> GMGEKLELRLKSPVGAEPAVYPWPLPVYDKHHDAAHEIIETIRWVCEEIPDLKLAMENYVLIDYDTKSFESMQRLCDKYNRAIDSIHQLWKGTTQPMKLNTRPSTGLLRHILQQVYNHSVTDPEKLNNYEPFSPEVYGETSFDLVAQMIDEIKMTDDDLFVDLGSGVGQVVLQVAAATNCKHHYGVEKADIPAKYAETMDREFRKWMKWYGKKHAEYTLERGDFLSEEWRE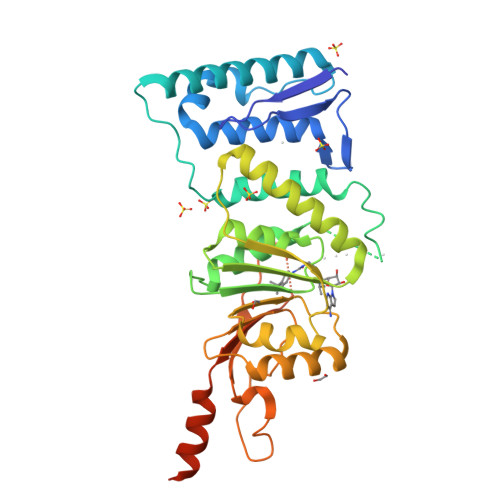RIANTSVIFVNNFAFGPEVDHQLKERFANMKEGGRIVSSKPFAPLNFRINSRNLSDIGTIMRVVELSPLKGSVSWTGKPVSYYLHTIDRTILENYFSSLKNPKLREEQEAARRRQQRESKS>GAMGRNDNGAIRVYASSTIGNYILPEIIARYRRDFPDLPLEMSVGNSLDVVQAVCDFRVDIGLIEGPCHMAEIVAQPWLEDELVVFASPASPLLEGEVTLERLAAMPWILREKGSGTREIVDYLLLSHLPQFRLSMELGNSEAIKHAVRHGLGVSCLSRRVIAEQLETGSLVEVKVP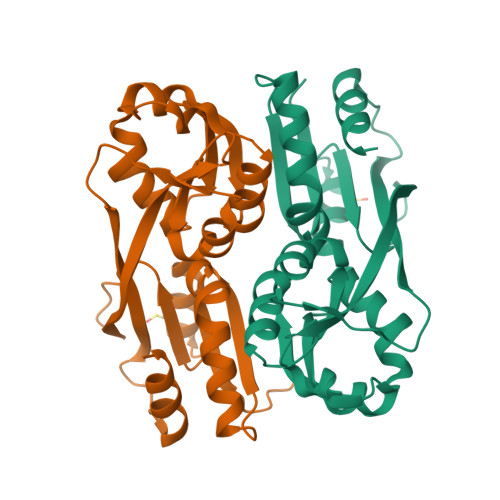LPPLVRTLYRIHHRQKHLSSALARFLRYCEL[2x]> MRPERLTVRNFLGLKNVDIEFQSGITVVEGPNGAGKSSLFEAISFALFGNGIRYPNSYDYVNRNAVDGTARLVFQFERGGKRYEIIREINALQRKHNAKLSEILENGKKAAIAAKPTSVKQEVEKILGIEHRTFIRTVFLPQGEIDKLLISPPSEITEIISDVFQSKETLEKLEKLLKEKMKKLENEISSGGAGGAGGSLEKKLKEMSDEYNNLDLLRKYLFDKSNFSRYFTGRVLEAVLKRTKAYLDILTNGRFDIDFDDEKGGFIIKDWGIERPARGLSGGERALISISLAMSLAEVASGRLDAFFIDEGFSSLDTENKEKIASVLKELERLNKV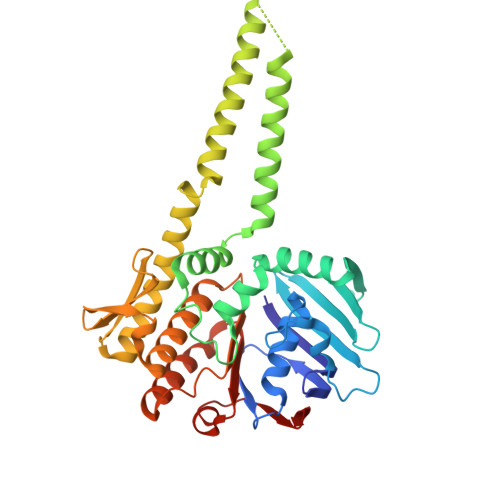IVFITHDREFSEAFDRKLRITGGVVVNE> KKV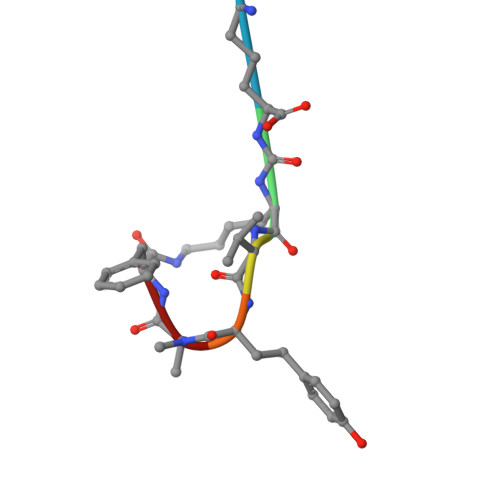YAF> QINQVRPKLPLLKILHAAGAQGEMFTVKEVMHYLGQYIMVKQLYDQQEQHMVYCGGDLLGELL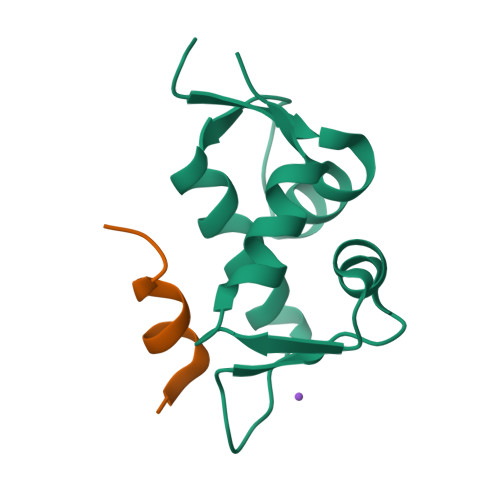GRQSFSVKDPSPLYDMLRKNLVTLAT;> LTFEHWWAQLTS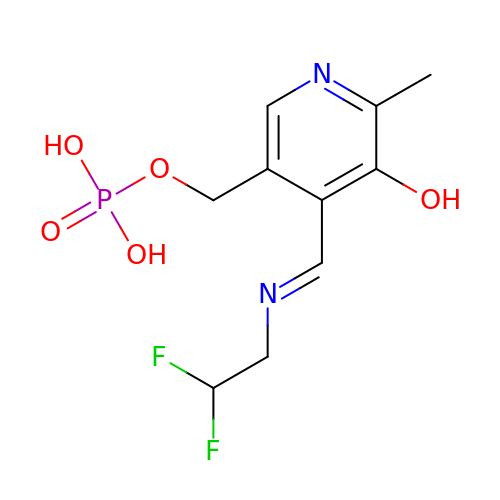(4-{(E)-[(2,2-DIFLUOROETHYL)IMINO]METHYL}-5-HYDROXY-6-METHYLPYRIDIN-3-YL)METHYL DIHYDROGEN PHOSPHATE | C10 H13 F2 N2 O5 P | OXVHZSPVJUCFDH-QLKAYGNNSA-N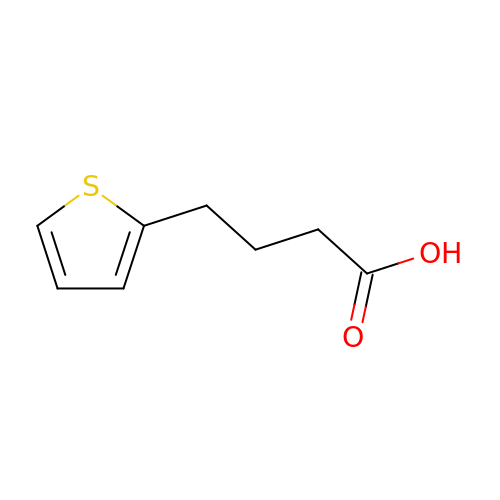4-(2-THIENYL)BUTYRIC ACID | C8 H10 O2 S | VYTXLSQVYGNWLV-UHFFFAOYSA-N> APRRLPIF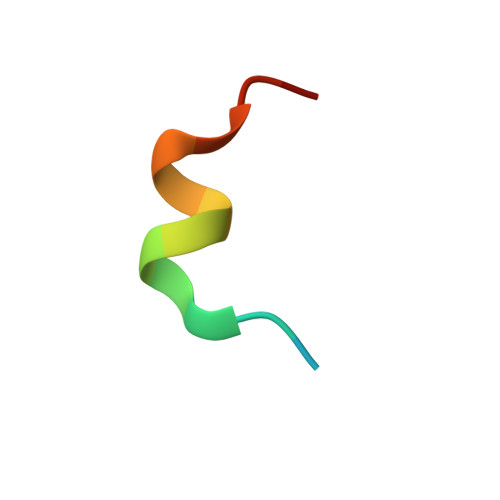NRISVSE> MQAAALLLLVLRAITSIEAAADDVNPDDNKEDFAVLCALAALANLQTTVPSIDTSGLAAYDNLQQLNLSLSSKEWKSLFNKAADSNGSPKQPPEGFQSDPTWRKQWPIWVTAAAALKAENKEAAVLARAGLTNAPEELRNRARLALIPLLAQAEQIRDRLSEIQKQNEDTTPTAIAKALNKAVYGQDKETGAVYNSADCFSGNVADSTQNSCKAGNQASKATTVAATIVCVCHKKNGGNDAANACGRLINHQSDAGANLATASSDFGDIIATCAARPPKPLTAAYLDSALAAVSARIRFKNGNGYLGKFKATGCTGSAAEGLCVEYTALTAATMQNFYKIPWVKEISNVAEALKRTEKDAAESTLLSTTLKASENQGNSVAQKLIKVGDSKAVPPAQRQTQNKPGSNCNKNLKKSECKDSDGCKWNRTEETEGDFCKPKETGTENPAAGTGEGAAGANTETKKCSDKKTEGDCKDGCKWDGKECKDSSILATKKFALTVVS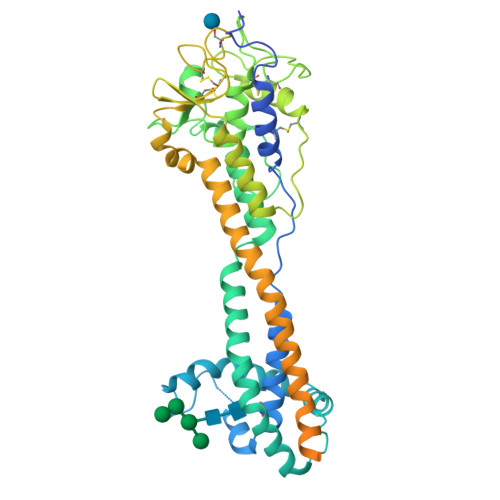AAFVALL> GPMSQVLFHQLVPLQVKCKDCEERRVSIRMSIELQSVSNPVHRKDLVIRLTDDTDPFFLYNL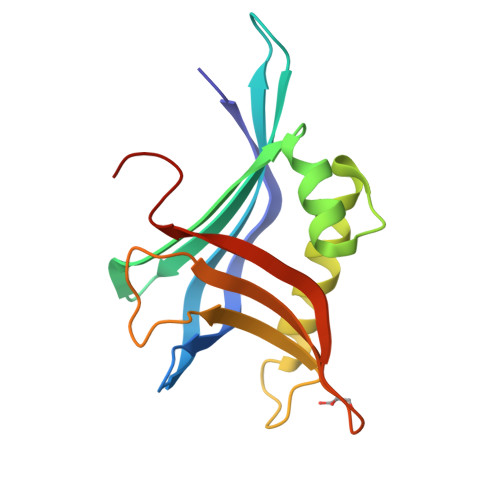VISEEDFQSLKFQQGLLVDFLAFPQKFIDLLQQCTQEHAKEIPRFLLQLVSPAAILDNSPAFLNVVETNPEKHLTHLSLKLLPGNDVEIKKF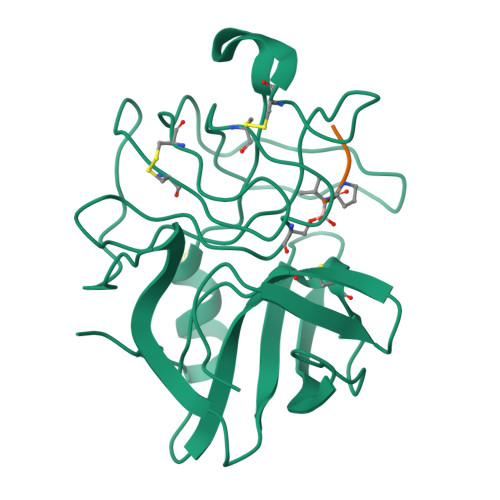> ANIVGGIEYSINNASLCSVGFSVTRGATKGFVTAGHCGTVNATARIGGAVVGTFAARVFPGNDRAWVSLTSAQTLLPRVANGSSFVTVRGSTEAAVGAAVCRSGRTTGYQCGTITAKNVTANYAEGAVRGLTQGNACAGRGDSGGSWITSAGQAQGVMSGGNVQSNGNNCGIPASQRSSLFERLQPILSQYGLSLVTG;> XAAPV> GAGS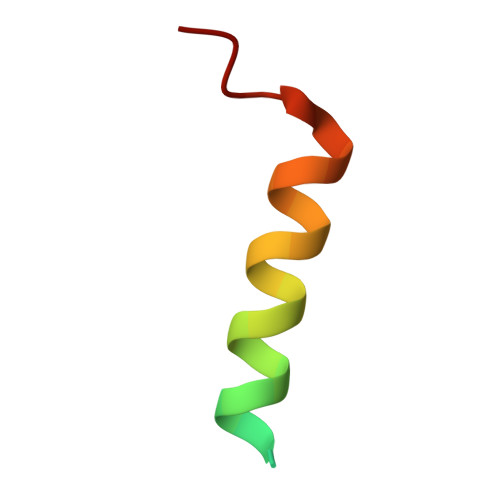GVTRFDEKQIEELLDNCIETFVAEKTT> TCGTCA;> 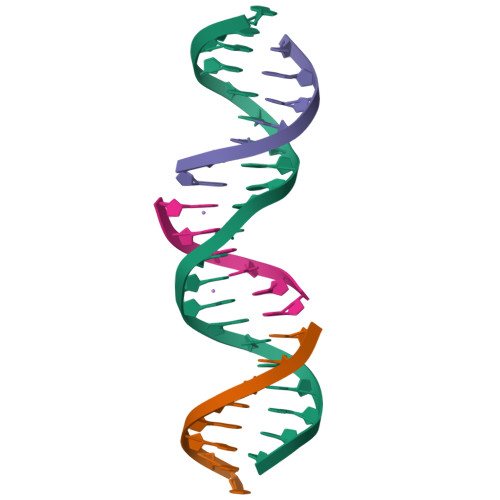GAACGACATTGACGAGGAGTC;> TCGAGTCC;> ATGTCGT> ESIESITDNYLFS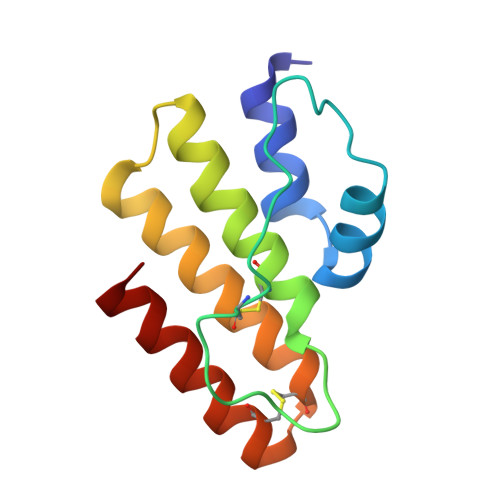TSPSQFEKVRDERPHADKLDWSSDSCSWAPDKPVGFDFDPACHRHDFGYRNYKKQSRFDDTSKKRIDDNFYSDLKGICHGNGSCNALAWTYYQAVRKFGS>[2x]MTIRNQRFSLLKQPISSTLNQHLVDYPTPSNLSYWWGFGSLAGICLVIQIVTGVFLAMHYTPHVDLAFNSVEHIMRDVEGGWLLRYMHANGASMFFIVVYLHIFRGLYYASYSSPREFVWCLGVVIFLLMIVTAFIGYVLPWGQMSFWGATVITSLASAIPVVGDTIVTWLWGGFSVDNATLNRFFSLHYLLPFILVGASLLHLAALHQYGSNNPLGVHSEMDKIAFYPYFYVKDLVGWVAFAIFFSIWIFYAPNVLGHPDNYIPANPMSTPPHIVPEWYFLPIYAILRSIPDKAGGVAAIALVFICLLALPFFKSMYVRSSSFRPIYQGMFWLLLADCLLLGWIGCQPVEAPFVTIGQISSLVFFLFFAITPILGRVGRGIPNSYTDETDHT;>MLRVAGRRLFSVSQRSSTATSFVVSRDHTLSDGGGDSSSAPRSLPSADLSSYHRSLIRGFSSQVLAQGNEIGFGSEVPAT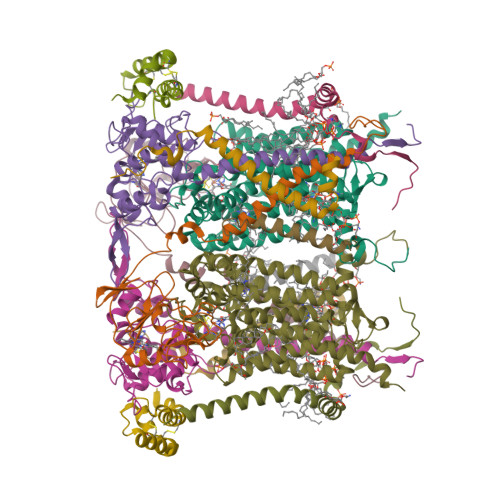VEAVKTPNSKIVYDDHNHERYPPGDPSKRAFAYFVLSGGRFVYASVLRLLVLKLIVSMSASKDVLALASLEVDLGSIEPGTTVTVKWRGKPVFIRRRTEDDIKLANSVDVGSLRDPQEDSVRVKNPEWLVVVGVCTHLGCIPLPNAGDYGGWFCPCHGSHYDISGRIRKGPAPYNLEVPTYSFLEENKLLIG[2x];>MVGGGVIRQLLRRKLHSQSVATPVLSWLSSKKANEDAGSAGLRAFALMGAGITGLLSFSTVASADEAEHGLECPNYPWPHEGILSSYDHASIRRGHQVYQQVCASCHSMSLISYRDLVGVAYTEEEAKAMAAEIEVVDGPNDEGEMFTRPGKLSDRLPEPYSNESAARFANGGAYPPDLSLVTKARHNGQNYVFALLTGYRDPPAGISIREGLHYNPYFPGGAIAMPKMLNDEAVEYEDGTPATEAQMGKDVVSFLSWAAEPEMEERKLMGFKWIFLLSLALLQAAYYRRLKWSVLKSRKLVLDVVN[2x];>MGKQPVKLKAVVYALSPFQQKIMTGLWKDLPEKIHHKVSENWISATLLVTPVVGTYWYAQYFKEQEKLEHRF[2x];>[2x]MADDEVVDPKKYLEESCKPKCVKPLLEYQACVKRIQGDDSGHKHCTGQYFDYWQCIDKCVAPKLFAKLK;>MEYAARRNQKGAFEGFYKLIMRRNSVYVTFIIAGAFFGERAVDYGVHKLWERNNVGKRYEDISVLGQRPVEE[2x];>[2x]MAGTSGLLNAVKPKIQTIDIQAAAGWGIAAAAGAIWVVQPFGWIKKTFIDPPPTEEK>[2x]SMGTKLKKSNNDITIFSENEYNEIVEMLRDYSNGDNLEFEVSFKNINYPNFMRITEHYINITPENKIESNNYLDISLIFPDK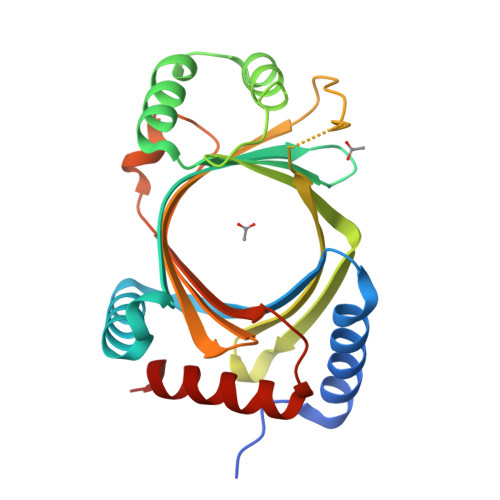NVYRVSLFNQEQIGEFITKFSKASSNDISRYIVSLDPSDDIEIVYKNRGSGKLIGIDNWAITIKSTEEIPLVAGKSKISKPKITGSERIMYRYKTRYSFTINKNSRIDITDVKSSPIIWKLMTVPSNYELELELINKIDINTLESELLNVFMIIQD> VPSPYLLSDKEVREIVQQSLSVGNFAARLLVRLFPELFTTENLRLQYNHSGACNKKQLDPTRLRLIRHYVEAVYPRAKNDRVWHYECIPSIDERCRRPN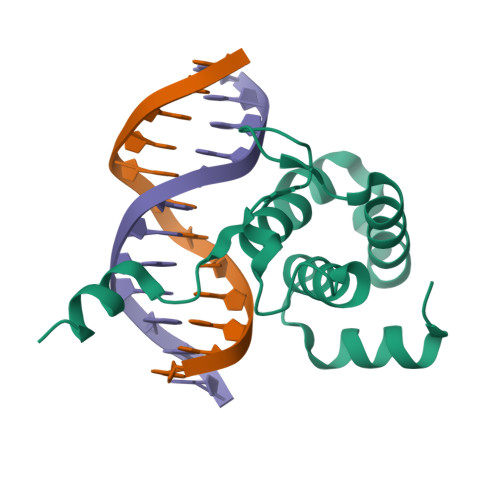RKKCDILKKAKKVEK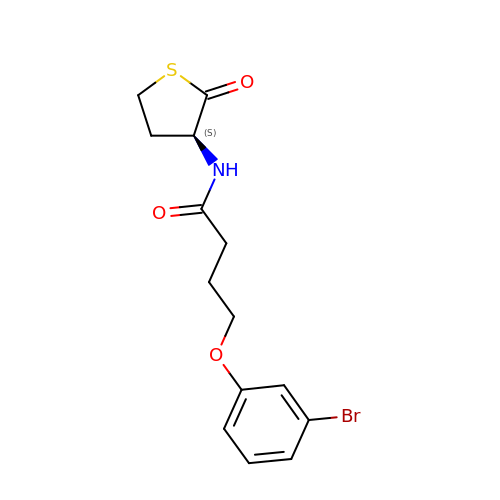4-(3-bromophenoxy)-N-[(3S)-2-oxothiolan-3-yl]butanamide | C14 H16 Br N O3 S | WTRVPDIAMVDWRQ-LBPRGKRZSA-N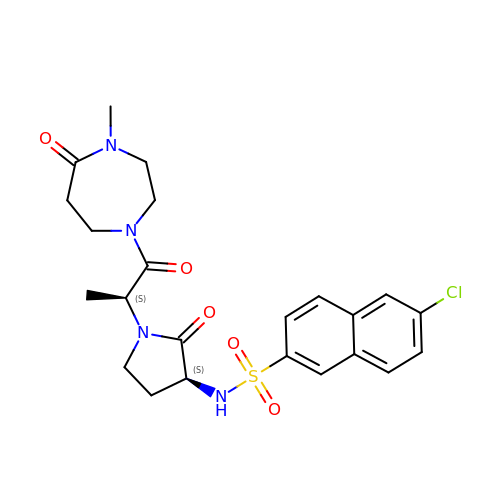6-chloro-N-{(3S)-1-[(2S)-1-(4-methyl-5-oxo-1,4-diazepan-1-yl)-1-oxopropan-2-yl]-2-oxopyrrolidin-3-yl}naphthalene-2-sulfonamide | C23 H27 Cl N4 O5 S | USQCUKQZXOWUDF-YWZLYKJASA-N>[4x]MNHHHHHHENLYFQGGAHMEEHYYVSIDIGSSSVKTIVGEKFHNGINVIGTGQTYTSGIKNGLIDDFDIARQAIKDTIKKASIASGVDIKEVFLKLPIIGTEVYDESNEIDFYEDTEI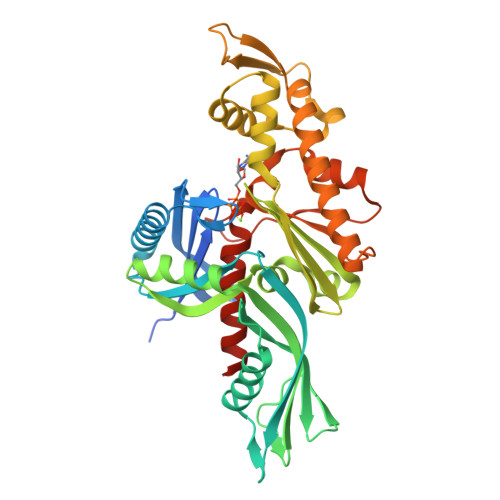NGSHIEKVLEGIREKNDVQETEVINVFPIRFIVDKENEVSDPKELIARHSLKVEAGVIAIQKSILINMIKCVEACGVDVLDVYSDAYNYGSILTATEKELGACVIDIGEDVTQVAFYERGELVDADSIEMAGRDITDDIAQGLNTSYETAEKVKHQYGHAFYDSASDQDIFTVEQVDSDETVQYTQKDLSDFIEARVEEIFFEVFDVLQDLGLTKVNGGFIVTGGSANLLGVKELLSDMVSEKVRIHTPSQMGIRKPEFSSAISTISSSIAFDELLDYVTINYH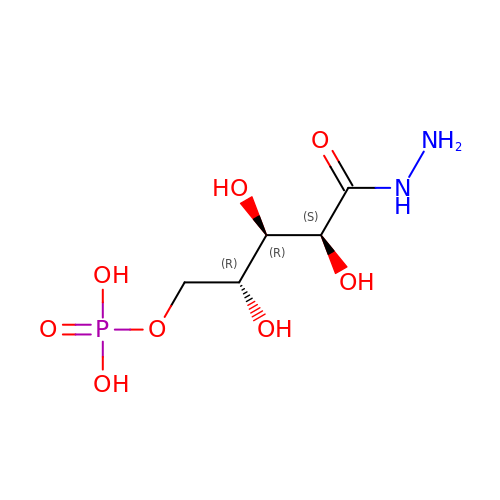[(2~{R},3~{R},4~{S})-5-diazanyl-2,3,4-tris(oxidanyl)-5-oxidanylidene-pentyl] dihydrogen phosphate | C5 H13 N2 O8 P | ZPAONOPLWIBTOD-JJYYJPOSSA-N> YAGTFAVLGGETEMPWAFDRLFRYEISDEMKKLQLTEDSKFRLTTNIIASNGSKVSNDIFPTPTVIFVPKKERTEQVSTTKSVRGNLVRKNVDRLSLQEINSLIHALKRMQKDRSSDGFETIASFHALPPLCPNPTAKHRHACCLH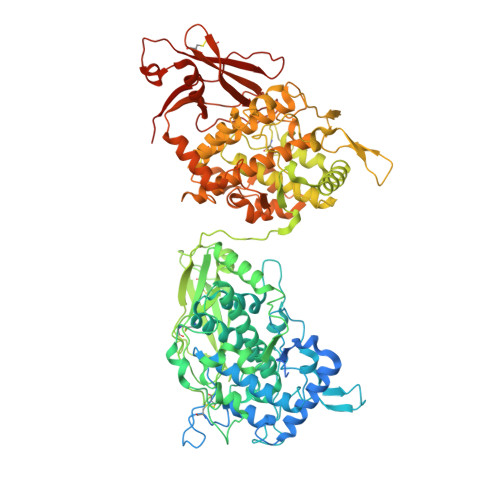GMATFPQWHRLYVVQFEHSLNRHGAIVGVPYWDWTYPMTEVPGLLTSEKYTDPFTGIETFNPFNHGHISFISPETMTTREVSEHLFEQPALGKQTWLFNNIILALEQTDYCDFEVQFEIVHNSIHSWLGGKELYSLNHLHYAAYDPAFFLHHSNVDRLWVVWQELQKFRGLPAYESNCAIELMSQPLKPFSFGAPYNLNPVTTKYSKPSDVFNYKQNFHYEYDMLEMNGMSIAQLESYIRQERQKDRVFAGFLLEGFGSSAYATFQVCPDVGDCYEGSHFSVLGGSTEMPWAFDRLYKMEITDILQAMALKFDSHFTIKTKIVAHNGTELPESLLPEATIVRIPPSAQNLEVAIPLNRIRRNINSLESRDVQNLMSALKRLKEDESDFGFQTIAGYHGSLMCPTPEAPEYACCLHGMPTFMHWHRVYLLHFEESMRRHGASVAVPYWDWTMPSDNLPSLLGDADYYDAWTDSVIENPFLRGHIKYEDTYTVREIQPELFALAEGQKESTLFKDVMLMFEQEDYCDFEVQAEVIHNSIHYLIGGHQKYAMSSLMFSSFDPIFYVHHSMVDRLWAIWQELQKHRKLPHDKAYCALDQMAFPMKPFIWESNPNPTTRAVSTPSKLFDYKSLGYDYDHLNFHGMSIGQLEALIQKQKKADRVFAGFLLHGIKISADVHLKICIEADCQEAGVIFVLGGETEMPWHFDRNYKMDITDVLKKRNIPPEALFEHDSKIRLEVEIKSVDGAVLDPNSLPKPSLIYAPAKGLIIQQVGEYDAG Non-homologous end joining (NHEJ) is the primary pathway for repairing DNA double-strand breaks (DSBs) in many organisms, including Mtb, where it is mediated by the Ku protein and the multifunctional LigD enzyme. The NHEJ mechanism in bacteria is a simplified system compared to the human counterpart, as it is reliant on the action of only two proteins: Ku and Ligase D (LigD). Multiple studies have shown the ability of Ku to bind double-stranded DNA ends, interact with LigD and stimulate LigD repair activities. In this study, we demonstrate that Ku is essential for mycobacterial survival under DNA-damaging conditions.

To determine the mechanistic details of Ku-Mtb biding to DNA, we added a DNA substrate containing a 32 bp double-strand and 20 nt single-strand (SS), previously utilised for UvrD1 and Ku studies. Following data processing we subsequently obtained a map to 2.96 Å resolution, into which we could model a filament of Ku-Mtb bound to DNA. This filament is continuous with a minimal repeating unit of two Ku-Mtb homodimers bound to one DNA duplex, in agreement with our EMSA experiments indicating a stable complex of four Ku protomers with 1 DNA duplex. Within our cryo-EM map, we have modelled 1.5 repeating units (3 Ku-Mtb homodimers and two DNA molecules). The central DNA binding cradle of Ku-Mtb threads on to DNA, in a similar manner to human Ku70/80. Neighbouring repeating units position the two DNA ends at a distance of ~40 Å apart. Given the high quality of the experimental map, we were able to visualise density corresponding to a potential metal ion (likely to be Mg due to MgCl2 in the buffer) coordinated by residues His27, Asp26, Asp28 from one protomer and Trp169, Glu172 from another protomer, which is at the interface between two Ku protomers but not within binding distance to the DNA substrate, therefore it is likely that this ion has a role in structural stability of the Ku homodimer. We observe direct Ku-Ku protein interfaces within the filament, which is formed by two α-helices and two intertwined loops forming a largely hydrophobic interface. Interestingly, within the DNA filament cryo-EM map, no density was observed for the C-terminal α-helix, as identified within the apo structure. Instead, it appears that the C-terminal helix has been displaced by either the action of DNA binding or the binding of Ku-Mtb at the filament interface.

>[6x]MAHHHHHHVGTGSNDDDDKSPDPMRAIWTGSIAFGLVNVPVKVYSATADHDIRFHQVHAKDNGRIRYKRVCEACGEVVDYRDLARAYESGDGQMVAITDDDIASLPEERSREIEVLEFVPAADVDPMMFDRSYFLEPDSKSSKSYVLLAKTLAETDRMAIVHFTLRNKTRLAALRVKDFGKREVMMVHTLLWPDEIRDPDFPVLDQKVEIKPAELKMAGQVVDSMADDFNPDRYHDTYQEQLQELIDTKLEGGQAFTAEDQPRLLDEPEDVSDLLAKLEASVKARSKANSNVPTPP>[2x]APAAVDWREKGAVTPVKDQGQCGSCWAFSTIGNIEGQWQVAGNPLVSLSEQMLVSCDTIDFGCGGGLMDNAF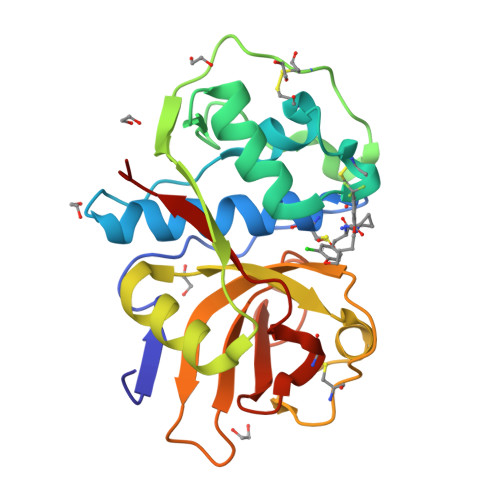NWIVNSNGGNVFTEASYPYVSGNGEQPQCQMNGHEIGAAITDHVDLPQDEDAIAAYLAENGPLAIAVDATSFMDYNGGILTSCTSEQLDHGVLLVGYNDASNPPYWIIKNSWSNMWGEDGYIRIEKGTNQCLMNQAVSSAVVGGP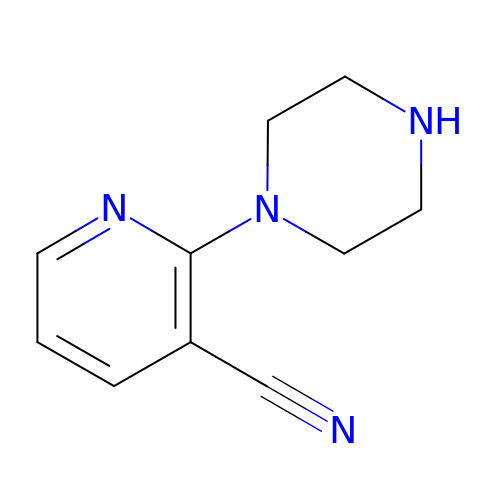2-(piperazin-1-yl)pyridine-3-carbonitrile | C10 H12 N4 | QSMNQUURWIAXAA-UHFFFAOYSA-N>RTIVVTTILESPYVMYKKNHEQLEGNERYEGYCVDLAYEIAKHVRIKYKLSIVGDGKYGARDPETKIWNGMVGELVYGRADIAVAPLTITLVREEVIDFSKPFMSLGISIMIKKGTPIESAEDLAKQTEIAYGTLDSGSTKEFFRRSKIAVYEK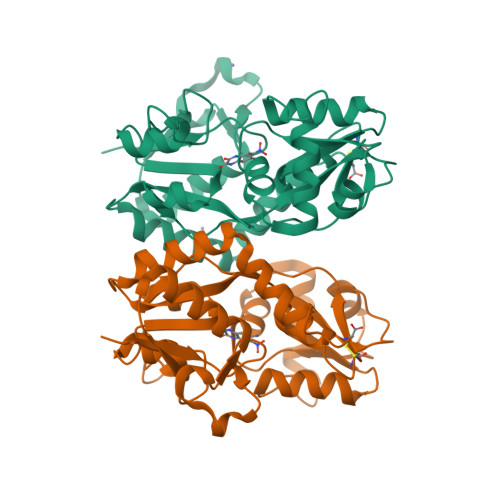MWSYMKSAEPSVFTKTTADGVARVRKSKGKFAFLLESTMNEYIEQRKPCDTMKVGGNLDSKGYGVATPKGSALGNAVNLAVLKLNEQGLLDKLKNKWWYDKGEC[2x]>[4x]MNYPAEPFRIKSVETVSMIPRDERLKKMQEAGYNTFLLN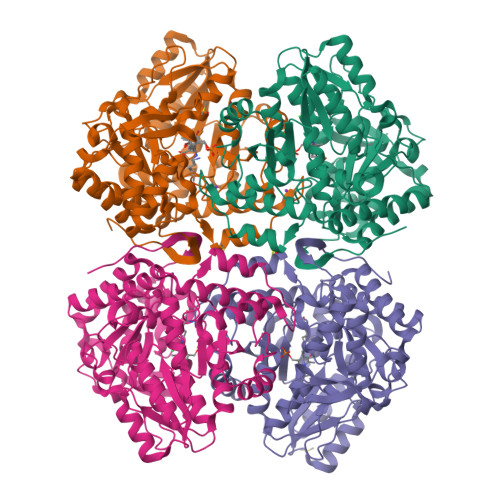SKDIYIDLLTDSGTNAMSDKQWAGMMMGDEAYAGSENFYHLERTVQELFGFKHIVPTHQGRGAENLLSQLAIKPGQYVAGNMYFTTTRYHQEKNGAVFVDIVRDEAHDAGLNIAFKGDIDLKKLQKLIDEKGAENIAYICLAVTVNLAGGQPVSMANMRAVRELTAAHGIKVFYDATRCVENAYFIKEQEQGFENKSIAEIVHEMFSYADGCTMSGKKDCLVNIGGFLCMNDDEMFSSAKELVVVYEGMPSYGGLAGRDMEAMAIGLREAMQYEYIEHRVKQVRYLGDKLKAAGVPIVEPVGGHAVFLDARRFCEHLTQDEFPAQSLAASIYVETGVRSAERGIISAGRNNVTGEHHRPKLETVRLTIPRRVYTYAHMDVVADGIIKLYQHKEDIRGLKFIYEPKQLRFFTARFDYI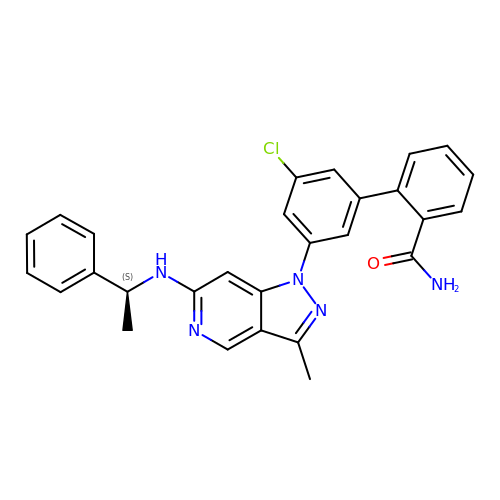3'-chloro-5'-(3-methyl-6-{[(1S)-1-phenylethyl]amino}-1H-pyrazolo[4,3-c]pyridin-1-yl)biphenyl-2-carboxamide | C28 H24 Cl N5 O | IFCBXJXWEYHVPY-KRWDZBQOSA-N> SVDHGFLVTRHSQTTDDPQCPPGTKILYHGYSLLYVQGNERAHGQDLGTAGSCLRKFSTMPFLFCNINNVCNFASRNDYSYWLSTPEPMPMSMAPITGENIR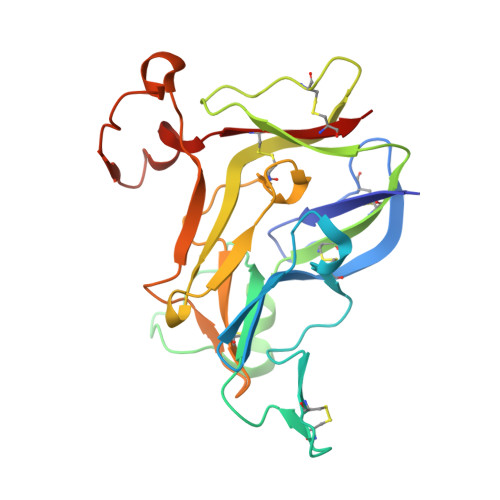PFISRCAVCEAPAMVMAVHSQTIQIPQCPTGWSSLWIGYSFVMHTSAGAEGSGQALASPGSCLEEFRSAPFIECHGRGTCNYYANAYSFWLATIERSEMFKKPTPSTLKAGELRTHVSRCQVCMRRT>MAGSYNYAEALQKAIYFYECQQAGPLPEWNRVEWRGDATMNDEVLGGWYDAGDHVKFNLPMAYSAAMLGWALYEYGDDIEASGQRLHLERNLAFALDYLVACDRGDSVVYQIGDGAADHKWWGSAEVIEKEMTRPYFVGKGSAVVGQMAAALAVGSIVLKNDTYLRYAKKYFELADATRSDSTYTAANGFYSSHSGFWDELLWASTWLYLATGDRNYLDKAESYTPKLNRQNQTTDIEYQWAHCWDDCHYGAMILLARATGKEEYHKFAQMHLDWWTPQGYNGKRVAYTPGGLAHLDTWGPLRYATTEAFLAFVYADSINDPALKQKYYNFAKSQIDYALGSNPDNRSYVVGFGNNPPQRPHHRTAHGTWLDKRDIPEKHRHVLYG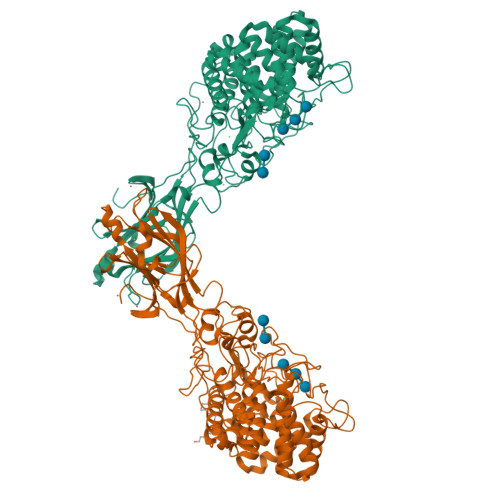ALVGGPGRDDSYEDNIEDYVKNEVACDYNAGFVGALCRLTAEYGGTPLANFPPPEQRDDEFFVEAAINQASDHFTEIKALLNNRSSWPARLIKDLSYNYYMDLTEVFEAGYSVDDIKVTIGYCESGMDVEISPITHLYDNIYYIKISYIDGTNICPIGQEQYAAELQFRIAAPQGTKFWDPTNDFSYQGLTRELAKTKYMPVFDGATKIFGEVPGGLEHHHHHH[2x]> ATCDDGRTTANAACCILFPILDDIQENLFDGAQCGEEVHESLRLTFHDAIGFSPTLGGGGADGSIIAFD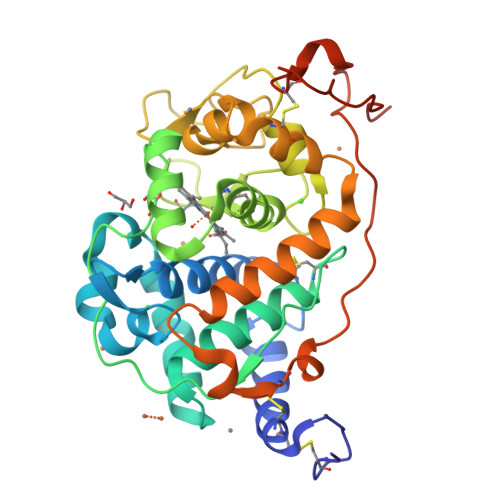TIETNFPANAGIDEIVSAQKPFVAKHNISAGDFIQFAGAVGVSNCPGGVRIPFFLGRPDAVAASPDHLVPEPQDSVDSILARMGDAGFSPVEVVWLLASHSIAAADKVDPSIPGTPFDSTPGVFDSQFFIETQLKGRLFPGTADNKGEAQSPLQGEIRLQSDHLLARDPQTACEWQSMVNNQPKIQNRFAATMSKMALLGQDKTKLIDCSDVIPTPPALVGAAHLPAGFSLSDVEQACAATPFPALTADPGPVTSVPPVPGS> MHHHHHHSSGRENLYFQGGSLLELQKKYHLKGAIGQGSYGVVRVAIENQTRAIRAIKIMNKNKIRQINPKDVERIKTEVRLMKKLHHPNIARLYEVYE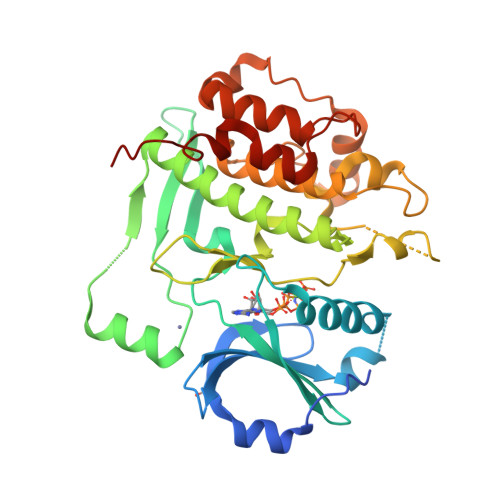DEQYICLVMELCHGGHLLDKLNVFIDDSTGKCAMDVVKTQICPCPECNEEAINGSIHGFRESLDFVQREKLISNIMRQIFSALHYLHNQGICHRDIKPENFLFSTNKSFEIKLVDFGLSKEFYKLNNGEYYGMTTKAGTPYFVAPEVLNTTNESYGPKCDAWSAGVLLHLLLMGAVPFPGVNDADTISQVLNKKLCFENPNYNVLSPLARDLLSNLLNRNVDERFDAMRALQHPWISQFSDKIYKMS>GSMPDYVAKYPVIQTDDEREAYKAVFQDQFSEYKELSAEVQAVLRKFDELDAVMSRLPHHSESRQEHEAISRIHEEFKKKKNDPTFLEKKERCDYLKNKLSHIKQRIQEYDKVMN[2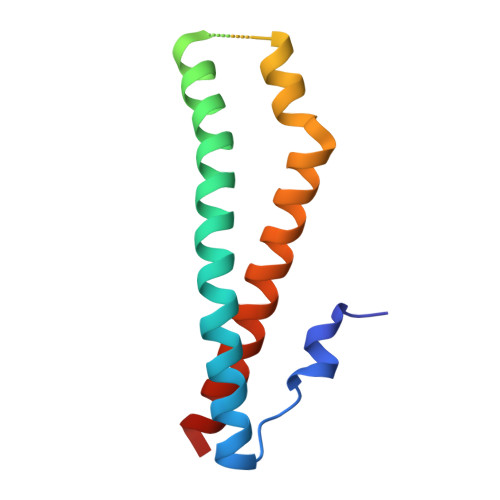x]>[2x]TVAYIAIGSNLASPLEQVNAALKALGDIPESHILTVSSFYRTPPLGPQDQPDYLNAAVALETSLAPEELLNHTQRIELQQGRV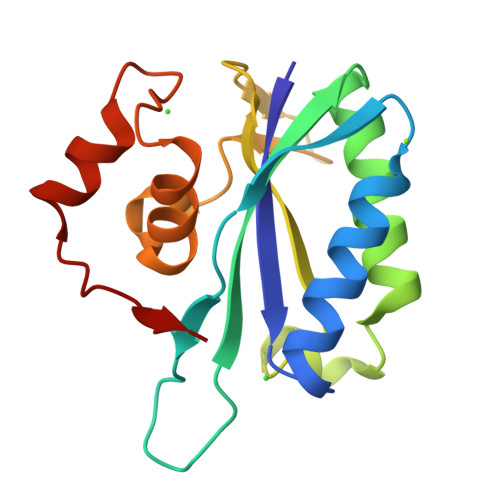RKAERWGPATLDLDIMLFGNEVINTERLTVPHYDMKNRGFMLWPLFEIAPELVFPDGEMLRQILHTRAFDKLNKW> MKDIAIRGYCDRPSVATGETIRFYVSANETRGTFDAELVRLIHGDSNPAGPGYKEEAIKSDLEGQYPARFQRTQFGSYVEVADPDAGLQPDGAFSVHLFLWSTTPSRGRQGIASRWNDERQSGWNLAIEDGRVVFTIGDGSGATSSVVSDRPLFQQIWYSITGVYDPEKKQLRLYQKSVVNRTNSRFGLVVPLDSDCAVSADATVKAADSETSLLIAGLGEAAAQDGRTWCIAHYNGKVDAPKIYGCALGQDDAEKLSRGEIVRPISRLAHWDFSAGIGLNGIPTDHVVDASGYGHHGRCMNQPSRGSTGWNWDGHEENFIHCPEQYGALWFHEDCLDDCRWEKDFEFTVPEGLKSDFYAVKIRYEDTEDYIPFFVLPPRGTATAPILVIASTLSYLAYANEQIMHKADIGQAVAGHTPVLNENDVELHKNLSYYGLSTYDGHIDGRGVQYTSWRRPIMNLRPKHRQGFGSIWELPADLHLIDWLNHNGFEYDVATEHDLNDQGAELLRRYKVVLTGS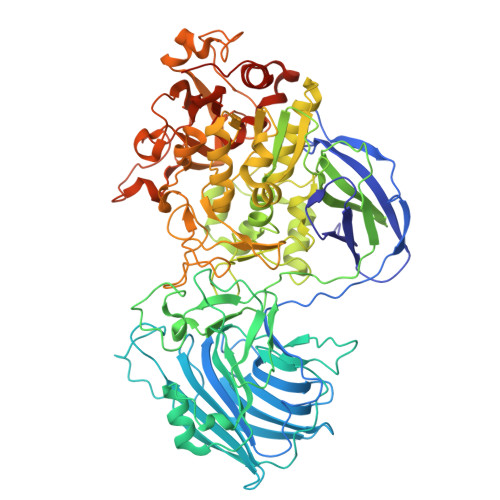HPEYQTWANADAWEDYLADGGRGMYLAANGMYWIVEVHPEKPWVMEVRKELGVTAWEAPPGEYHYSTNGRRGGRFRGRARATQKIWGTGMSSFGFDHSGYFVQMPDSQDERVAWIMEGIDPEERIGDGGLVGGGAGGYELDRYDLALGTPPNTLLLASSVEHSVVYTVIPDDKAFPHPGMNGGEHPFVRADITYFSTANGGGMFATSSISWLGSLSWNDYDNNVSKMTKNVLNQFIKDEPAPRVKLAAALEHHHHHH>GAIIFSAKDIFEQEFGREVRGYNKVEVDEFLDDVIKDYETYAALVKSLRQEIADLKEELTRK[2x];>[2x]TILRRSRSDRKKLA

GpsB has emerged as a major regulator of PG biosynthesis in low G+C Gram-positive bacteria, and its homologues (DivIVA/Wag31/antigen 84) in Actinobacteria play essential roles in hyphal growth and branching. To gain molecular understanding of GpsB function, we report three crystal structures of PBP cytoplasmic mini-domains in complex with GpsB, the first structures of a PG synthase in complex with a cytoplasmic cell cycle regulator. The PG synthase arginine finger pokes into a negatively charged cavity situated between α-helices 1 and 2 of GpsB and is fixed in the same orientation in all structures, just as the phosphoryl group defines the binding orientation of peptides to 14-3-345. Therefore, the role of GpsB in the bacterial cell cycle is that of an adaptor, docking PG synthases to other cell wall enzymes, scaffolds and shape determinants into protein complexes for division (the divisome) and peripheral growth (the elongasome).

Synthetic lethality studies in pneumococcal ΔgpsB suppressor mutants revealed that pbp1a, and not pbp2a, became essential in the absence of gpsB indicating that SpPBP2a is the class A PBP regulated by SpGpsB in S. pneumoniae. We found that the cytoplasmic mini-domain of SpPBP2a and many of its orthologues contain the consensus sequence (S/R)RS(R/G)(K/S)xR that resembles the Bacillaceae PBP1 SRxxR(R/K) motif. In this instance, each subunit of the SpGpsB dimer is peptide-bound. Peptide binding principally involves two arginines but each SpGpsB subunit recognises the peptide differently. The importance of SpPBP2aArg31 and SpPBP2aArg33 is further supported by their sequence conservation and FP. Although SpPBP2aArg31Lys had only a 2-fold reduced affinity, which probably reflects the ability of SpPBP2aArg33 to compensate for the loss of SpPBP2aArg31, the binding affinity of SpPBP2aArg31Lys,Arg33Lys was reduced >25-fold relative to wild type. The arginine complements the cavity best when the mainchain amide protons of it and its downstream residue are accessible to form hydrogen bonds with BsGpsBAsp35, LmGspBAsp37 or SpGspBAsp33. This scenario can occur when the arginine is either at the start of an α-helix, such as BsPBP1Arg8, or at the i + 1 position in a type I β turn, such as SpPBP2aArg31, which explains why free l-arginine does not displace pre-bound PBP peptides from GpsB even when present at 100-fold molar excess. The interaction was lost completely with SpGpsBTyr23Ala, SpGpsBVal28Ala, SpGpsBAsp29Ala, SpGpsBLeu32Ala and SpGpsBAsp33Ala mutated proteins and reduced with SpGpsBIle36Ala.>MTPPHNYLAVIKVVGIGGGGVNAVNRMIEQGLKGVEFIAINTDAQALLMSDAD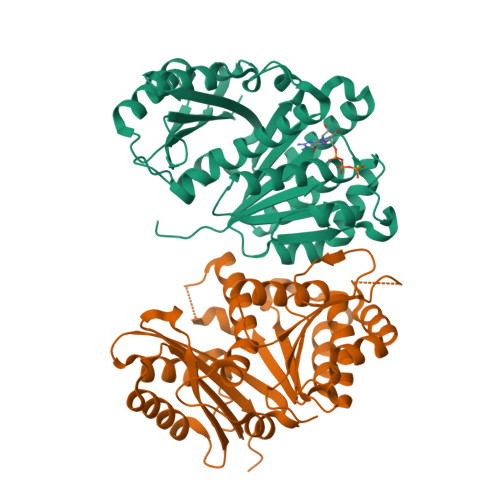VKLDVGRDSTRGLGAGADPEVGRKAAEDAKDEIEELLRGADMVFVTAGEGGGTGTGGAPVVASIARKLGALTVGVVTRPFSFEGKRRSNQAENGIAALRESCDTLIVIPNDRLLQMGDAAVSLMDAFRSADEVLLNGVQGITDLITTPGLINVDFADVKGIMSGAGTALMGIGSARGEGRSLKAAEIAINSPLLEASMEGAQGVLMSIAGGSDLGLFEINEAASLVQDAAHPDANIIFGTVIDDSLGDEVRVTVIAAGFDVS[2x]> DVSGTVCLSALPPEATDTLNLIASDGPFPYSQDGVVFQNRESVLPTQSY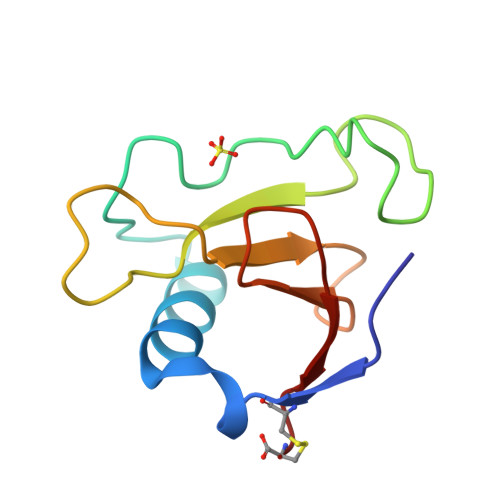GYYHEYTVITPGARTRGTRRIITGEATQEDYYTGDHYATFSLIDKTC>[2x]MSL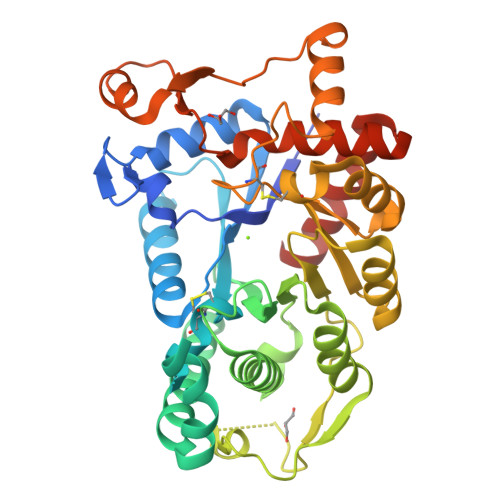TSTATDSPLKYYDIGLNLTDPMFHGIYNGKQYHPADYVKLLERAAQRHVKNALVTGSSIAESQSAIELVSSVKDLSPLKLYHTIGVHPCCVNEFADASQGDKASASIDNPSMDEAYNESLYAKVISNPSFAQGKLKELYDLMNQQAKPHDTSFRSIGEIGLDYDRFHYSSKEMQKVFFEEQLKISCLNDKLSSYPLFLHMRSACDDFVQILERFVVGFTDEKDTFQLQKLGASSSSGFYKFHPDRKLVVHSFTGSAIDLQKLLNLSPNIFIGVNGCSLRTEENLAVVKQIPTERLLLETDAPWCEIKRTHASFQYLAKYQEVRDFEYPAFKSVKKNKLADKLNAEELYMVKGRNEPCNMEQVAIVVSEVKDVDLATLIDTTWKTTCKIFGEGHHHHHH> MRCVGISNRDFVEGLSATGWVDVVLEHGSCVTTMAKDKPTLDIELLKTEVTNPAILRKLCIEAKISNTTTDSRCPTQGEATLVEEQDTNFVCRRTFVDRGWGNGCGLFGKGSLITCAKFKCVTKLEGKIVQYENLKYSVIVTVHTGDQHQVGNETTEHGTTATITPQAPTSEIQLTDYGALTL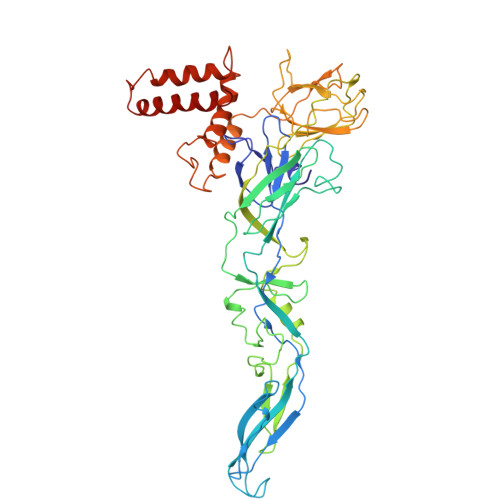DCSPRTGLDFNEMVLLTMKEKSWLVHKQWFLDLPLPWTSGASTSQETWNRQDLLVTFKTAHAKKQEVVVLGSQEGAMHTALTGATEIQTSGTTTIFAGHLKCRLKMDKLTLKGVSYVMCTGSFKLEKEVAETQHGTVLVQVKYEGTDAPCKIPFSSQDEKGVIQNGRLITANPIVTDKEKPVNIEAEPPFGESYIVVGAGEKALKLSWFKKGSSIGKMFEATARGARRMAILGDTAWDFGSIGGVFTSVGKLVHQIFGTAYGVLFSGVSWTMKIGIGILLTWLGLNSRSTSLSMTCIAVGMVTLYLGVMVQA> GEIAAIKQE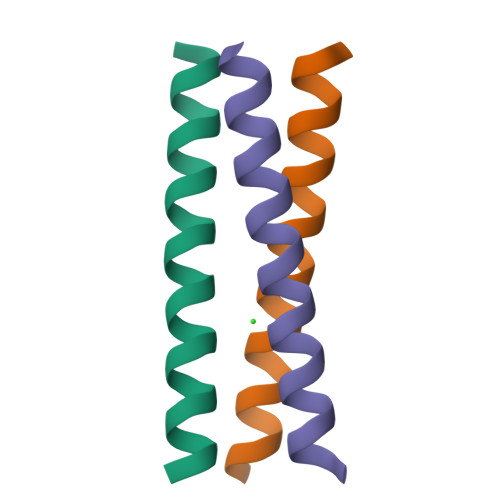IAANKKEIAAIKWEIAAIKQGYG> ANPCCSNPCQNRGECMSTGFDQYKCDCTRTGFYGENCTTPEFLTRIKLLLKPTPNTVHYILTHFKGVWNIVNNIPFLRSLIMKYVLTSRSYLIDSPPTYNVHYGYKSWEAFSNLSYYTRALPPVADDCPTPMGVKGNKELPDSKEVLEKVLLRREFIPDPQGSNMMFAFFAQHFTAQFFKTDHKRGPGFTRGLGHGVDLNHIYGETLDRQHKLRLFKDGKLKYQVIGGEVYPPTVKDTQVEMIYPPHIPENLQFAVGQEVFGLVPGLMMYATIWLREHQRVCDILKQEHPEWGDEQLFQTSKLILIGETIKIVIEDYVQHLSGYHFKLKFDPELLFNQQFQYQNRIASEFNTLYHWHPLLPDTFNIEDQEYS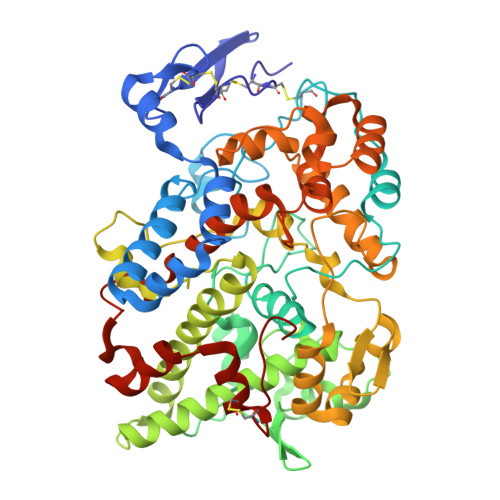FKQFLYNNSILLEHGLTQFVESFTRQIAGRVAGGRNVPIAVQAVAKASIDQSREMKYQSLNEYRKRFSLKPYTSFEELTGEKEMAAELKALYSDIDVMELYPALLVEKPRPDAIFGETMVELGAPFSLKGLMGNPICSPQYWKPSTFGGEVGFKIINTASIQSLICNNVKGCPFTSFNVQ>[2x]TPEMPVLENRAAQGDITAPGGARRLTGDQTAALRDSLSDKPAKNIILLIGDGMGDSEITAARNYAEGAGGFFKGIDALPLTGQYTHYALNKKTGKPDYVTDSAASATAWSTGVKTYNGALGVDIHEKDHPTILEMA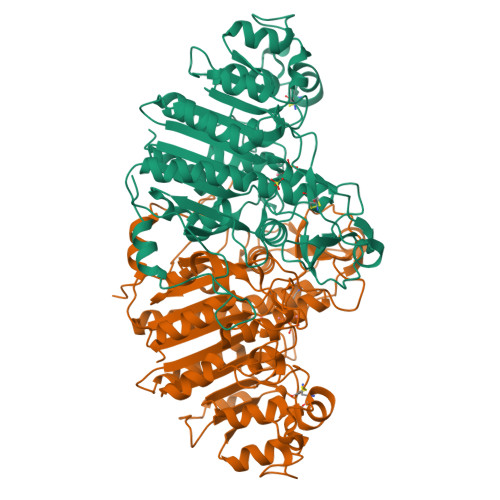KAAGLATGNVSTAELQDATPAALVAHVTSRKCYGPSATSEKCPGNALEKGGKGSITEQLLNARADVTLGGGAKTFAETATAGEWQGKTLREQAQARGYQLVSDAASLNSVTEANQQKPLLGLFADGNMPVRWLGPKATYHGNIDKPAVTCTPNPQRNDSVPTLAQMTDKAIELLSKNEKGFFLQVEGASIDKQDHAANPCGQIGETVDLDEAVQRALEFAKKEGNTLVIVTADHAHASQIVAPDTKAPGLTQALNTKDGAVMVMSYGNSEEDSQEHTGSQLRIAAYGPHAANVVGLTDQTDLFYTMKAALGLK> UCCCAGUCCACCGU;> CGGUGAGAXGGGXGGCAGAGAA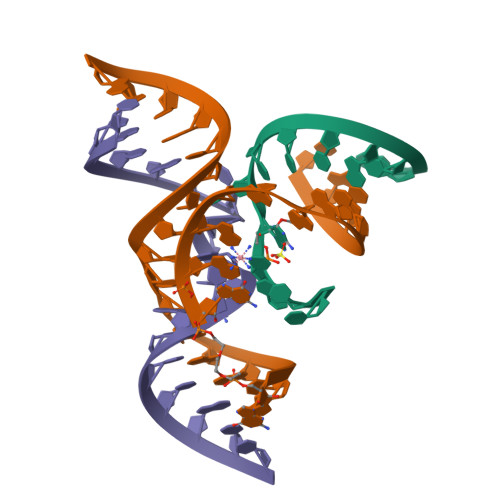ACACACGA;> UCGUGGUACAUUACCUGCC>MNKRIVTTALALATLLGVALLSGCQDVSTELKAPKYKTGIAETET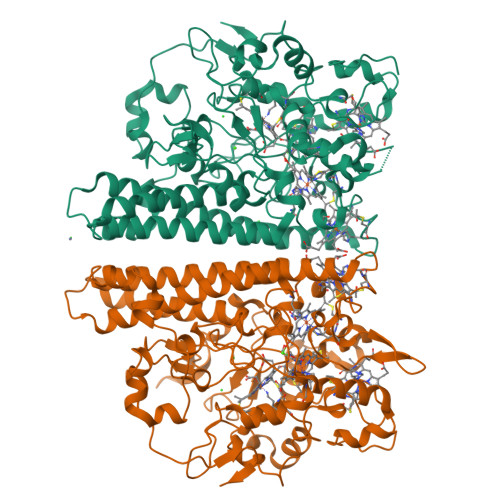KMSAFKGQFPQQYASYMKNNEDRIMTDYKGSVPYHKNDNVNPLPKGFKHAQPYLKNLWLGYPFMYEYNETRGHTYAIDDFLNIDRINRFAADGKGNLPATCWNCKTPKMMEWVSQYGDKFWSMDVNEFRAKDKINAHDETIGCANCHDPATMELRLYSEPLKDWLKRSGKDWQKMSRNEKRTLVCAQCHVEYYFTHKDNGPAAKPVFPWDNGFNPEDMYQYYKGHGAKGPDGKPGPFVDWVHAASKVPMIKMQHPEYETFQDGPHGAAGVSCADCHMQYVREDGKKISSHWMTSPMKDPEMRACRQCHADKTGEYLRQRVLYTQQKTFDQLLKAQEMSVKAHEAVRLANAYEGHRAANYEALMAEAREMVRKGQLFWDYVSAENSVGFHNPAKALDTLMTSMECSQKAVDLATEATDFGIAPALAGDIKKLVPPILTLSRKLQQDPEFLKQNPWTRLLPALPKAEQVWEGQDRA[2x]> TTSGWVKQDGAWYYFDGNGNLVKNAWQGSYYLKADGKMAQSEWIYDSSYQAWYYLKSDGSYAKNAWQGAYYLKSNGKMAQGEWVYDSSYQAWYYLKSDGSYARNAWQGNYYLKSDGKMAKGEWVYDATYQAWYYLTSDGSYAYSTWQGNYYLKSDGKMAVNEWVDGGRYYVGADGVWKEVQA

Here, we describe the functional characterization and the three-dimensional structure of CbpL from S. pneumoniae. The functional protein has 3 well-differentiated domains connected by linker regions that provide flexibility to the general structure. Taken together, these results indicate that CbpL is a CBP non-covently attached to the phosphorylcholine of pneumococcal teichoic acids. Our studies indicated that CbpL plays a critical role both in pneumococcal lung infections and in transmigration from nasopharynx to the lungs and blood, therefore pointing to a direct role of CbpL in host-pathogen interactions.

Crystallization trials with full-length CbpL systematically resulted in proteolysis of the sample through the linker regions and only the choline-binding module (CbpLCBM) was incorporated into the crystals. The crystal structure presents three residues of the N-term linker (Thr92-Ser94), the CBM that is composed of nine choline-binding repeats (residues Gly95-Glu270), and three more residues from the C-term linker (Val271-Ala273). The overall shape of the CbpLCBM is approximately a triangular prism of 81 Å high and 22 Å side with the choline-binding sites placed along the three lateral faces of the prism. CbpLCBM is folded in a left-handed superhelical arrangement of the choline-binding repeats, each of them comprising a β-hairpin followed by a loop and a coiled region that is linked to the next repeat, as previously reported in other CBPs15161726. The β-hairpin units stack along the structure (from N to C-terminal end) following a 120° counterclockwise rotation in such a way that choline-binding sites are formed at the interface of two consecutive β-hairpins. Instead, the repeats can be grouped in two main classes: the long repeats (21 to 23 residues-long; R1, R3, R5, R7 and R9) and the short repeats (17 residues-long; R2, R4, R6, R8). The crystal structure of CbpLCBM:choline complex shows that eight choline-binding sites are available. Among them, four are canonical sites (CS), displaying the typical choline stabilization found in other CBPs, while the other four are non-canonical sites (NCS). Remarkably, CS and NCS alternate along the CbpLCBM starting from a CS formed between R1 and R2 repeats. Due both to the repetitive pattern of CS and NCS sites along the CbpLCBM and the conservation of critical CbpL residues involved in TA recognition, up to four RU of TA can wrap around the CBM in a vine-like fashion.> SNA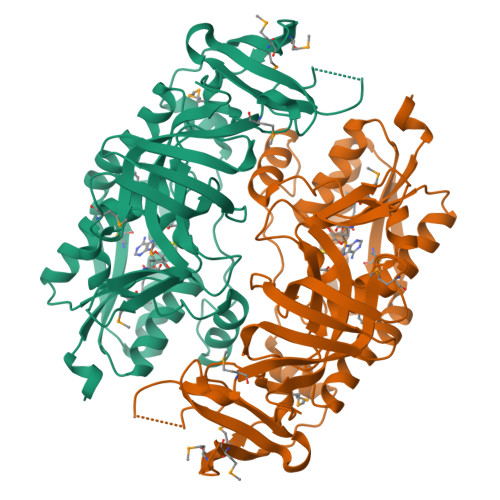MSDNSKTRVVVGMSGGVDSSVTALLLKEQGYDVIGIFMKNWDDTDENGVCTATEDYKDVVAVADQIGIPYYSVNFEKEYWDRVFEYFLAEYRAGRTPNPDVMCNKEIKFKAFLDYAITLGADYVATGHYARVARDEDGTVHMLRGVDNGKDQTYFLSQLSQEQLQKTMFPLGHLEKPEVRRLAEEAGLSTAKKKDSTGICFIGEKNFKNFLSNYLPAQPGRMMTVDGRDMGEHAGLMYYTIGQRGGLGIGGQHGGDNAPWFVVGKDLSKNILYVGQGFYHDSLMSTSLEASQVHFTREMPEEFTLECTAKFRYRQPDSKVTVHVKGEKTEVIFAEPQRAITPGQAVVFYDGEECLGGGLIDNAYRDGQVCQYI>MRGSHHHHHHTDPTGATFPEEAIADLSVNMYNRLRATGEDENILFSPLSIALAMGMMELGAQGSTQKEIRHSMGYDSLKNGEEFSFLKEFSNMVTAKESQYVMKIANSLFVQNGFHVNEEFLQMMKKYFNAAVNHVDFSQNVAVANYINKWVENNTNNLVKDLVSPRDFDAATYLALINAVYFKGNWKSQFRPENTRTFSFTKDDESEVQIPMMYQQGEFYYGEFSDGSNEAGGIYQVLEIPYEGDEISMMLVLSRQEVPLATLEPLVKAQLV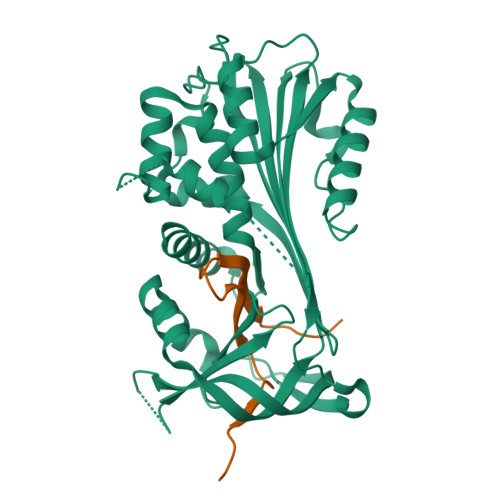EEWANSVKKQKVEVYLPRFTVEQEIDLKDVLKALGITEIFIKDANLTGLSDNKEIFLSKAIHKSFLEVNEEGSEAAAVSGMIAISR[2x];>[2x]MAVLYPQVIVDHPFFFLIRNRRTGTILFMGRVMHPETMNTSGHDFEEL>[2x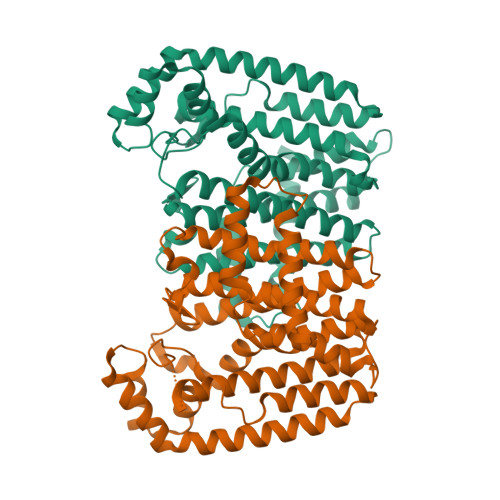]MNHKVHHHHHHIEGRHMSDLKSKFLEVYSVLKSELLNDPAFDFTDDSRLWVERMLDYNVPGGKLNRGLSVIDSFKLLKEGKEPTDEEIFLACVLGWCIEWLQAYFLVLDDIMDSSHTRRGQPCWFRLPKVGMIAVNDGLILRNHIPRILKKHFKGKPYYVDLLDLFNEVEFQTASGQMIDLITTLVGEKDLSKYSLPLHHRIVQYKTAYYSFYLPVACALVMSGENLDNHVDVKNILVEMGTYFQVQDDYLDCFGDPKFIGKIGTDIEDFKCSWLVVKALELANDEQKKLLHENYGKEDPECVAKVKKLYETLNLQDVFGEYERQSHGKLIKAIEGHSNKAVQFVLKSSLEKIYQRQK>[12x]MKEVIFTENAPKPIGP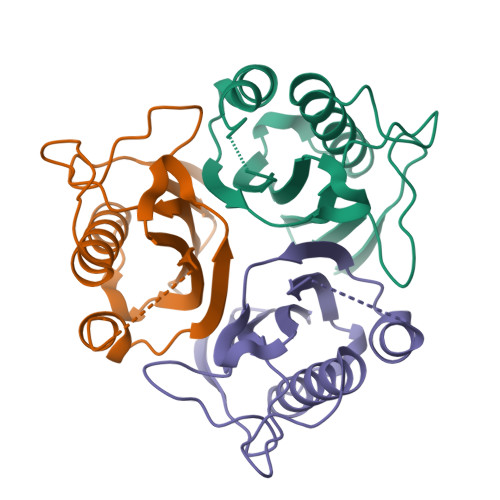YSQAIKAGNFLFIAGQIPIDPKTGEIVKGDIKDQTRQVLENIKAILEAAGYSLNDVIKVTVYLKDMNDFAKMNEVYAEYFGESKPARVAVEVSRLPKDVLIEIEAIAYKE> ATFEIVNRCSYTVWAAASKGDAALDAGGRQLNSGESWTINVEPGTNGGKIWARTDCYFDDSGSGICKTGDCGGLLRCKRFGRPPTTLAEFSLNQYGKDYIDISNIKGFNVPMDFSPTTRGCRGVRCAADIVGQCPAKLKAPGGGCNDACTVFQTSEYCCTTG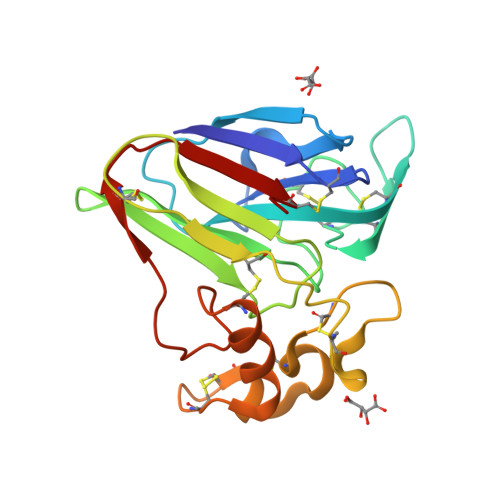KCGPTEYSRFFKRLCPDAFSYVLDKPTTVTCPGSSNYRVTFCPT>[10x]MEKFRAVLDLHVKHHSALGYGLVTLLTAGGERIFSAVAFQCPCSAAWNLPYGLVFLLVPALALFLLGYVLSARTWRLLTGCCSSARASCGSALRGSLVCTQISAAAALAPLTWVAVALLGGAFYECAATGSAAFAQRLCLGRNRSCAAELPLVPCNQAKASDVQDLLKDLKAQSQVLGWILIAVVIIILLIFTSVTRCLSPVSFLQLKFWKIYLEQEQQILKSKATEHATELAKENIKCFFEGSHPKEYNTPSMKEWQQISSLYTFNPKGQYYSMLHKYVNRKEKTHSIRSTEGDTVIPVLGFVDSSGINSTPEL

In humans, the CALHM family encompasses six paralogs, some of which function as non-selective channels that are permeable to large substances such as ATP. We identified the three paralogs, CALHM2, 4 and 6, to be highly expressed in this organ. The CALHM subunits thus constitute unique modular building blocks that assemble with different stoichiometries into large membrane channels. In contrast to previously described CALHM structures, where the oligomeric state of individual channels was described as uniform, our data show heterogeneous populations with CALHM4 and CALHM6 assembling as decameric and undecameric channels with similar abundance and CALHM2 as predominantly undecameric proteins with a smaller population of dodecamers (Figure 3—figure supplements 2–4 and 6). Despite the unknown activating stimuli, our study has provided insight into gating transitions of CALHM channels by showing two conformations with either a cylindrical pore of uniform large dimeter within the membrane that is constricted at the intracellular side as in case of CALHM4 and a conical pore that continuously narrows from its extracellular entry towards the cytoplasm as in case of CALHM6.

As in case of CALHM4, data of CALHM6 shows a heterogeneous distribution of decameric and undecameric channels, but in this case with a prevalence of the former amounting to 60% of the classified particles. Both assemblies of CALHM6 contain subunits with equivalent conformations, which are better defined in the smaller oligomers. We have thus chosen the decameric CALHM6 structure for a description of the conical pore of a CALHM channel. Unlike CALHM4, the lower resolution of the CALHM6 density of 4.4 Å, precludes a detailed interpretation of the structure for all parts of the protein. Unlike CALHM4, there is no dimerization of CALHM6 channels and the C-terminal region following the cytoplasmic helix CTH instead appears to engage in intramolecular interactions with the outside of the cytoplasmic rim for most of its length. Upon comparison of decameric channels of both paralogs, in CALHM6 we find a slight expansion of the protein parallel to the membrane and an accompanying moderate contraction in perpendicular direction. In a superposition of the subunits, similar conformations are observed for α-helices TM2 and 4 and the C-terminal helix CTH and larger differences in the interacting helices TM1 and 3. These differences are most pronounced for TM1, which in CALHM6 has detached from TM3 and moved by 60° towards the pore axis around a hinge located upstream of a conserved phenylalanine at the end of TM1. When viewed from the outside this transition thus resembles the closing of an aperture and it converts a cylindrical pore to a funnel which narrows towards the intracellular side while creating a large cavity between TM1 and TM3 that becomes accessible from the cytoplasm.> GACCTGT;> CGGACAGCATCGCA;> ACACCG;> TCTGCGATGC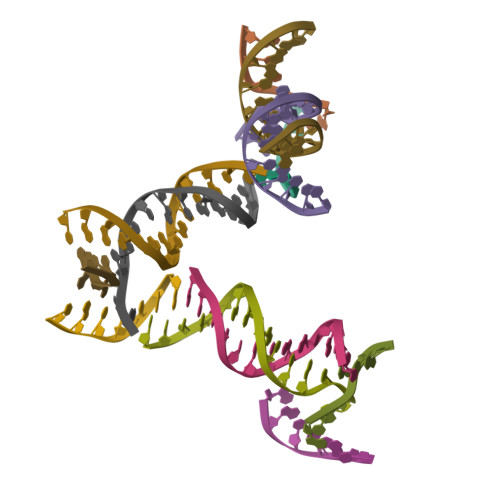TGTGG>[2x]MHHHHHHLVPRGSMFKKVLVANRGEIACRVIRACKELGIQTVAIYNEIESTARHVKMADEAYMIGVNPLDTYLNAERIVDLALEVGAEAIHPGYGFLAENEHFARLCEEKGITFIGPHWKVIELMGDKARSKEVMKRAGVPTVPGSDGILKDVEEAKRIAKEIGYPVLLKASA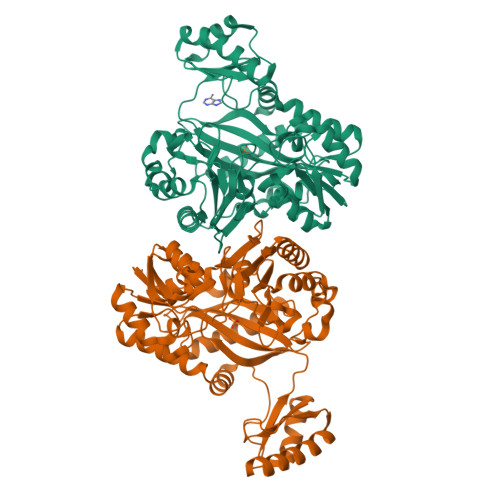GGGGRGIRISRNEEELVRNYENAYNEAVKAFGRGDLLLEKYIENPKHIEFQVLGDKYGNVIHLGERDCSIQRRNQKLVEIAPSLLLTPEQREYYGSLVVKAAKEIGYYSAGTMEFIADEKGNLYFIEMNTRIQVEHPVTEMITGVDIVKWQIRIAAGERLRYSQEDIRFNGYSIECRINAEDPKKGFAPSIGTIERYYVPGGFGIRVEHASSKGYEITPYYDSLIAKLIVWAPLWEVAVDRMRSALETYEISGVKTTIPLLINIMKDKDFRDGKFTTRYLEEHPHVFDYAEHRDKEDFVAFISAVIASYHGL> GPGSDNKEQTTDQPLAKDKVALLIGNMNYREHPKLKAPLVDVYELTNLLRQLDFKV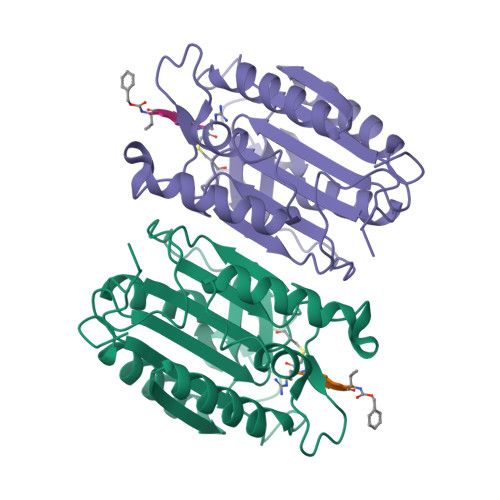VSLLDLTEYEMRNAVDEFLLLLDKGVYGLLYYAGHGYENFGNSFMVPVDAPNPYRSENCLCVQNILKLMQEKETGLNVFLLDMCRKRNDYDDTIPILDALKVTANIVFGYATCQGAEAFEIQHSGLANGIFMKFLKDRLLEDKKITVLLDEVAEDMGKCHLTKGKQALEIRSSLSEKRALTDPIQGTEY>[2x]MYGNWGRFIRVNLSTGDIKVEEYDEELAKKWLGSRGLAIYLLLKEMDPTVDPLSPENKLIIAAGPLTGTSAPTGGRYNVVTKSPLTGFITMANSGGYFGAELKFAGYDAIVVEGKAEKPVYIYIKDEHIEIRDASHIWGKKVSETEATIRKEVGSEKVKIASIGPAGENLVKFAAIMNDGHRAAGRGGVGAVMGSKNLKAIAVEGSKTVPIADKQKFMLVVREKVNKLRNDPVAGGGLPKYGTAVLVNIINENGLYPVKNFQTGVYPYAYEQSGEAMAAKYLVRNKPCYACPIGCGRVNRLPTVGETEGPEYESVWALGANLGINDLASIIEANHMCDELGLDTISTGGTLATAMELYEKGHIKDEELGDAPPFRWGNTEVLHYYIEKIAKREGFGDKLAEGSYRLAESYGHPELSMTVKKLELPAYDPRGAEGHGLGYATNNRGGCHIKNYMISPEILGYPY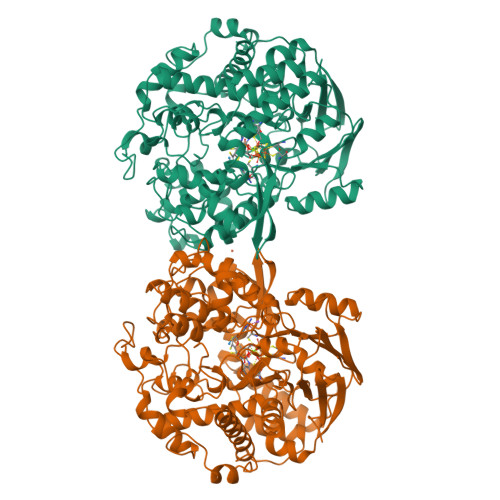KMDPHDVSDDKIKMLILFQDLTALIDSAGLCLFTTFGLGADDYRDLLNAALGWDFTTEDYLKIGERIWNAERLFNLKAGLDPARDDTLPKRFLEEPMPEGPNKGHTVRLKEMLPRYYKLRGWTEDGKIPKEKLEELGIAEFY>MPDDAKTANTTTAATTKNAENNRITPVTVIGLGAMGRALAGALLDAGYPTTVWNRTAGRGEDLVARGATLAASPAEAVRAGEVVLVCVVDYAASQAILEPVAADLAGRVLVNVTSDSPERAREAAKWADGHGIRYLDGAVMIPTVMVGSTDALLFYAGDKSAYDEHEQVFTSLGGQSAYVGADHGLAAVYELSMIDFFWTSMSGLVHGYALAAKDGVPATSIAPFL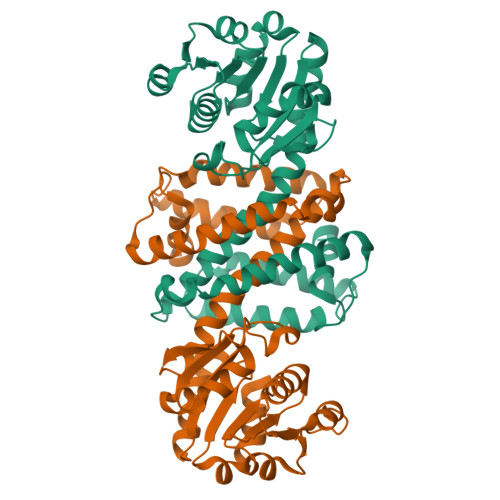KAHISLLSLLIEVTAKDLDAGEYPGAEGNLAMEVEGIEHILHAAELRGLDVSVLRSVRDVARRAVDLGHGADSWSATVEGARNPA[2x]>[2x]MYIGIDLGT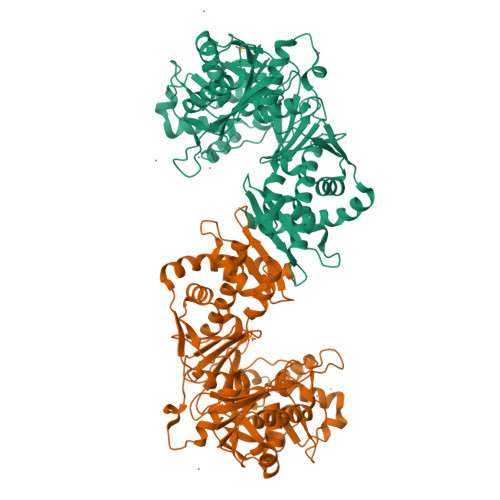SGVKVILLNEQGEVVAAQTEKLTVSRPHPLWSEQDPEQWWQATDRAMKALGDQHSLQDVKALGIAGQMHGATLLDAQQRVLRPAILWNDGRCAQECTLLEARVPQSRVITGNLMMPGFTAPKLLWVQRHEPEIFRQIDKVLLPKDYLRLRMTGEFASDMSDAAGTMWLDVAKRDWSDVMLQACDLSRDQMPALYEGSEITGALLPEVAKAWGMATVPVVAGGGDNAAGAVGVGMVDANQAMLSLGTSGVYFAVSEGFLSKPESAVHSFCHALPQRWHLMSVMLSAASCLDWAAKLTGLSNVPALIAAAQQADESAEPVWFLPYLSGERTPHNNPQAKGVFFGLTHQHGPNELARAVLEGVGYALADGMDVVHACGIKPQSVTLIGGGARSEYWRQMLADISGQQLDYRTGGDVGPALGAARLAQIAANPEKSLIELLPQLPLEQSHLPDAQRYAAYQPRRETFRRLYQQLLPLMA> HMKELKYDVLIIGGGFAGSSAAYQLSRRGLKILLVDSKPWNRIGDKPCGDAVSKAHFDKLGMPYPKGEELENKINGIKLYSPDMQTVWTVNHEGFELNAPLYNQRVLKEAQDRGVEIWDLTTAMKPIFEDGYVKGAVLFNRRTNEELTVYSKVVVEATGYSRSFRSKLPPELPITEDLDDKDADVAYREVLLTKEDIEDHDYLRIFIDQETSPGGYWWYFPKGKNKVNVGLGIQGGMGYPSIHEYYKKYLDKYAPDVDKSKLLVKGGALVPTRRPLYTMAWNGIIVIGDSGFTVNPVHGGGKGSAMISGYCAAKAILSAFETGDFSASGLWDMNICYVNEYGAKQASLDIFRRFLQKLSNDDINYGMKKKIIKEEDLLEASEKGDLHLSVADKAMRVISGLGRPSLLFKLKAVAESMKKIKELYLNYPRSPSSL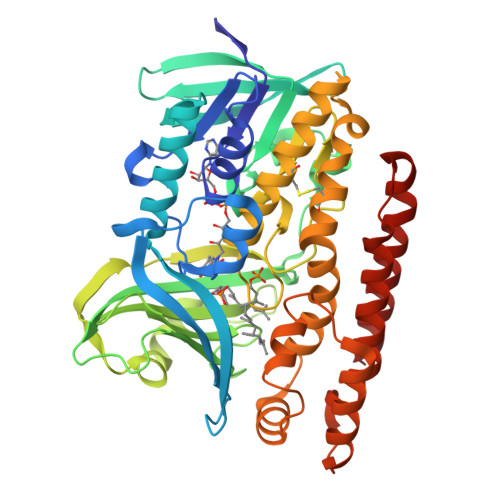GSWRREVDNVLTEFNKSLS> MASSYSASAEPARVRALVYGHHGDPAKVVELKNLELAAVRGSDVRVKMLAAPINPSDINMIQGNYGLLPELPAVGGNEGVAQVVAVGSNVTGLKPGDWVIPANAGLGTWRTEAVFSEEALIQVPSDIPLQSAATLGVNPCTAYRMLMDFEQLQPGDSVIQNASNSGVGQAVIQIAAALGLRTINVVRDRPDIQKLSDRLKSLGAEHVITEEELRRP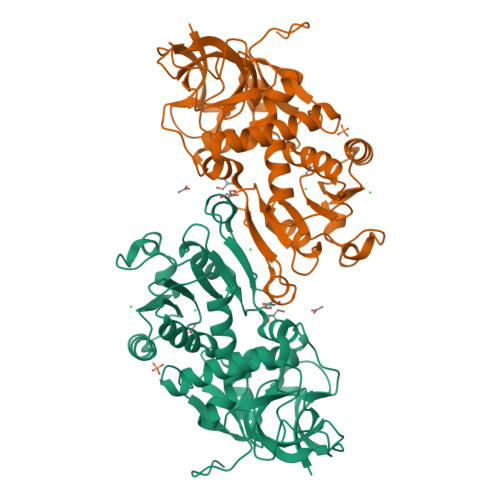EMKNFFKDMPQPRLALNCVGGKSSTELLRQLARGGTMVTYGGMAKQPVVASVSLLIFKDLKLRGFWLSQWKKDHSPDQFKELILTLCDLIRRGQLTAPACSQVPLQDYQSALEASMKPFISSKQILTMLEHHHHHH The coat proteins (CPs) of single-stranded RNA bacteriophages (ssRNA phages) directly assemble around the genomic RNA (gRNA) to form a near-icosahedral capsid with a single maturation protein (Mat) that binds the gRNA and interacts with the retractile pilus during infection of the host. The canonical ssRNA phage Qβ has a genomic RNA (gRNA) of 4217 nucleotides, from the 5′ to the 3′ end, encoding the maturation protein (Mat); the major coat protein (CP); the minor capsid protein A1, which is a read-through extension caused by a leaky stop codon for the major CP; and the β-subunit of the RNA-dependent RNA replicase (Rep). Like many other viruses, the CPs of ssRNA phages can also assemble into virus-like particles (VLPs), which are not infectious. Through a native infection without engineering the amino acid sequences, we found that Qβ CP can form diverse VLP capsids, including the T = 3 icosahedral, T = 4 icosahedral, prolate, oblate, and a small prolate form elongated along the 3-fold axis.

Recently, T = 4 capsids have been observed when overexpressing the covalently-linked CP dimers in ssRNA phages PP7 and MS2. Here, we have observed under normal wild-type phage infection, T = 4 capsids are also made, albeit a small percentage (0.5%) of the overall number of particles. The elongated faces of the small prolate consist of two triangulation numbers, Q1 = 2 and Q2 = 3. Figure 3A shows the five forms of the VLPs from the wild-type Qβ, each containing 240, 210, 180, 150, and 132 CP copies for the T = 4, prolate, T = 3, oblate, and small prolate forms, respectively. Though all of the 5 forms contain 12 copies of the pentamers, they consist of 30, 25, 20, 15, and 12 copies of the hexamers for the T = 4, prolate, T = 3, oblate, and small prolate forms, respectively. For the T = 3 and T = 4 VLPs, both are formed by only one type of hexamer. The T = 4 capsid has one type of hexamer with a θ angle of ~170°, defined as a “less arched” type.

>MAKLETVTLGNIGKDGKQTLVLNPRGVNPTNGVASLSQAGAVPALEKRVTVSVSQPSRNRKNYKVQVKIQNPTACTANGSCDPSVTRQAYADVTFSFTQYSTDEERAFVRTELAALLASPLLIDAIDQLNPAY[4x]Many proteins, including the EP300/CBP histone acetyltransferases (HATs), contain several targetable domains. EP300 and CBP broadly regulate the activity of other proteins through their protein acetyltransferase catalytic activity. These proteins contain several highly homologous domains, including KIX, bromodomains (BRDs) and HAT domains, through which they interact with, dock to, and acetylate target proteins, respectively. EP300/CBP are critical gene-regulatory targets in cancer, with existing high potency inhibitors of either the catalytic HAT domain or protein-binding bromodomain (BRD). Using crystallography, we identify the binding mechanism of the EP300/CBP-specific BRD inhibitor CCS1477 in complex with the EP300, CBP and BRD4 BRDs, and define components of the CCS1477 catalytic binding core that are required for compound activity.

Since recombinant CBP BRD was more robust in biochemical assays and crystallization studies, Kd values were determined for all compound-CBP interactions by MST, and co-crystal structures of the CBP BRD with five of the seven analogues were determined. Notably, replacement with a dihydrobenzodioxine moiety (compound 7) maintained high binding affinity (Kd = 17 nM), and the cocrystal structure confirmed unimpeded positioning and interaction with R1173. While none of the analogues were superior to CCS1477 in terms of binding affinity, substitutions were well tolerated if productive interactions with R1173 were maintained.

> KKIFKPEELRQALMPTLEALYRQDPESLPFRQPVDPQLLGIPDYFDIVKNPMDLSTIKRKLDTGQYQEPWQYVDDVWLMFNNAWLYNRKTSRVYKFCSKLAEVFEQEIDPVMQSLG> MSFREQDIYLPIANVARIMKNAI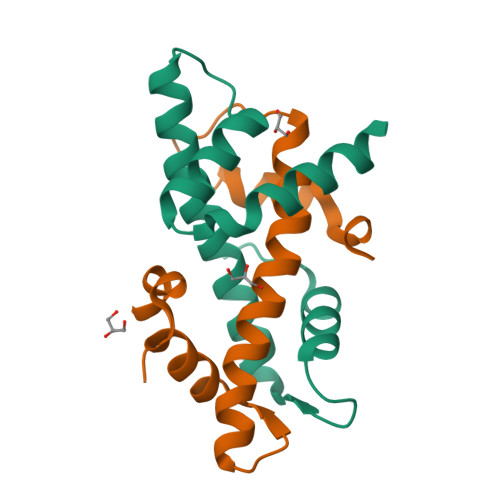PQTGKIAKDAKECVQECVSEFISFITSEASERCHQEKRKTINGEDILFAMSTLGFDSYVEPLKLYLQKFRE;> MEEIRNLTVKDFRVQELPLARIKKIMKLDEDVKMISAEAPVLFAKAAQIFITELTLRAWIHTEDNKRRTLQRNDIAMAITKFDQFDFLIDIVPR>MGHHHHHHTKVISKRKTILDTALSLFKQYSFKFVGVDRIINESQVAKMTFYKHFPSKTLLIQACLCEEQKTIEESILNELSLLSEAGNIARLKALLNWHVAYINQQNFNGCLFQKAVYENEVSEEVLSVIQAHKQWKFKLVSDLMEVPECCTAFVSSSMVYSMLEGMLLPANINPCVDHETAIKN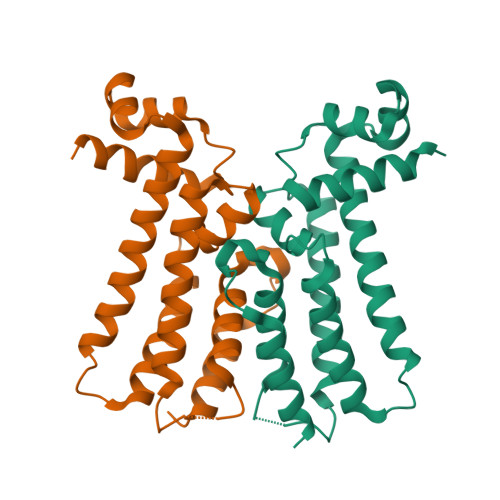LIQTFEA[2x]>SFDCGKPQVEPKKCPGRVVGGCVAHPHSWPWQVSLRTRFGMHFCGGTLISPEWVLTAAHCLEKSPRPSSYKVILGAHQEVNLEPHVQEIEVSRLFLEPTRKDIALLKLSSPAVITDKVIPACLPSPNYVVADRTECFITGWGETQGTFGAGLLKEAQLPVIENKVCNRYEFLNG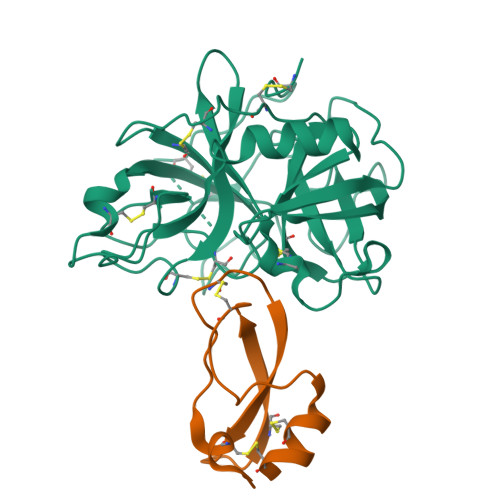RVQSTELCAGHLAGGTDSCQGDSGGPLVCFEKDKYILQGVTSWGLGCARPNKPGVYVRVSRFVTWIEGVMRNN[2x];>[2x]KDRPDFCELPADTGPCRVRFPSFYYNPDEKKCLEFIYGGCEGNANNFITKEECESTCAA>[2x]GSLRPLSEVNQHSQL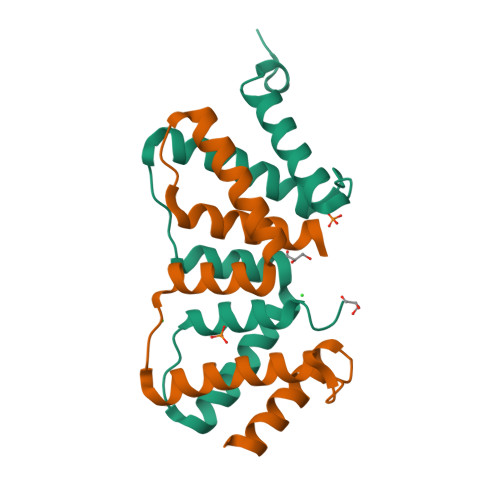MAQLVEVIEDSFQMKVNKESVNYLRLIRHIRFTIERIKKEEPTKEPEKLMLLLKNEYPLCYNTAWKLIKILQQTLKKPVHEAEAVYLTLHLIPINQ>GAGTMVKQIESKTAFQKALKAAGDKLVVVDFSATWCGPCKMIKPFFHSLSEKYSNVIFLEVDVDDCQDVASECEVKCMPTFQFFKKGQKVGEFSGANKKKLEATI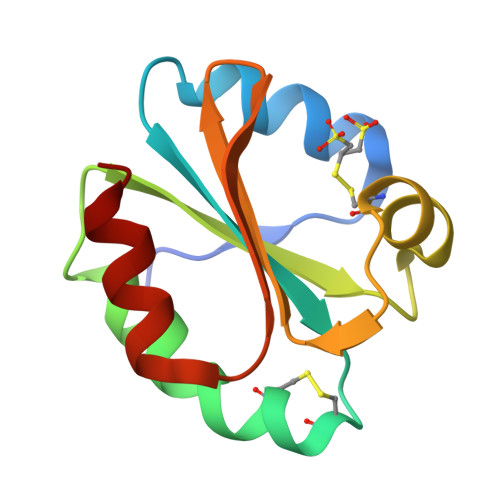NKLV[4x]> SKGKLGEKISQFKIVEELKAKGLYAYFRPIQSKQDTEVKIDGRRVLMFGSNSYLGLTTDTRIIKAAQDALEKYGTGCAGSRFLNGTLDIHVELEEKLSAYVGKEAAILFSTGFQSNLGPLSCLMGRNDYILLDERDHASIIDGSRLSFSKVIKYGHNNMEDLRAKLSRLPEDSAKLICTDGIFSMEGDIVNLPELTSIANEFDAAVMVDDAHSLGVIGHKGAGTASHFGLNDDVDLIMGTFSKSLASLGGFVAGDADVIDFLKHNARSVMFSASMTPASVASTLKALEIIQNEPEHIEKLWKNTDYAKAQLLDHGFDLGATESPILPIFIRSNEKTFWVTKMLQDDGVFVNPVVSPAVPAEESLIRFSLMATHTYDQIDEAI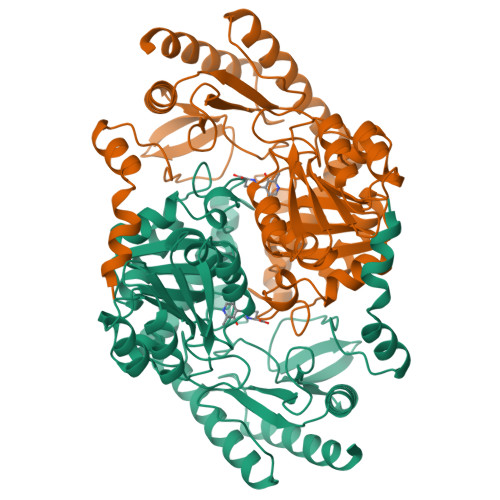EKMVKVFKQAEVETLI> VPATRILLLVLAVIIYGTAGFHFIEGESWT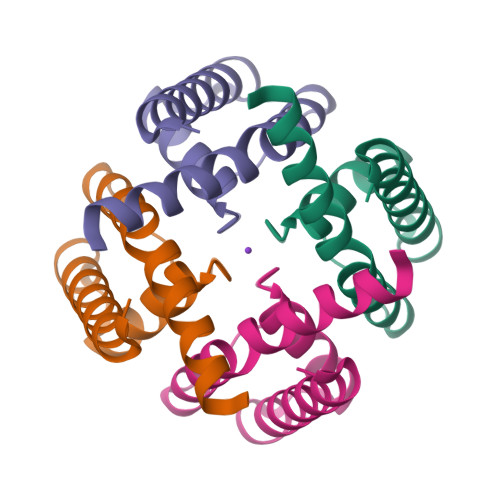VSLYWTFVTIATVGYGDYSPRTPLGMYFTCTLIVLGIGTFAVAVERLLEFLI> MKESVRFLTDFGEISDAISDLLTSSPNFNVISAIGPQGAGKSTLLSMLAGNNSRQMYREYVFRPVSREANEQSRHQTIQIDIYIVNHQIFLDCQPMYSFSIMEGLPKVRGGRFDDSTAMSDTLRLTAFLLYVSHTVLVVSETHYDKVIIDTLRVAEQIRPYLAIFRPKLAIDRKTNLVFIKTKASSIDLAPTVIREREELLRLSFQDSRWLKVSQEPFKTLIVLEEIRVRREHLFEEGDEPDEAASLNEFDEQIAELREELQKNREDFTVETAAMDEKKWLDMCREVIRDKTLHKTLKEY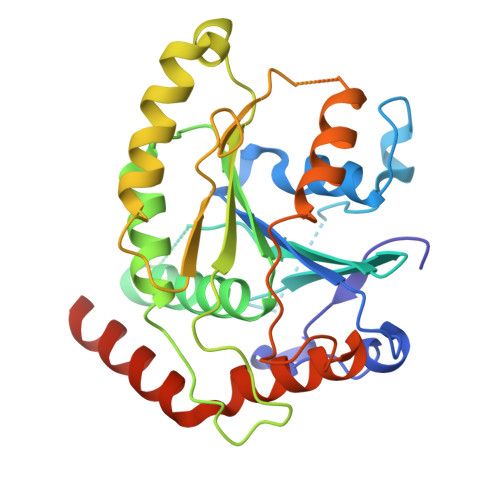QRAMTDGVRTHFDNGFH IDE can effectively degrade insulin, amylin, and glucagon, pancreatic hormones that control blood glucose levels, as well as amyloid β (Aβ), a peptide implicated in Alzheimer’s disease. IDE is a 110 kDa zinc metalloprotease that readily dimerizes in solution (Kd =~ 10 nM). IDE has at least two major conformational states in its catalytic cycle; open-state IDE captures substrates and releases products while closed-state IDE performs catalysis. Within the IDE dimer, each IDE subunit consists of ~55 kDa N- and C-terminal domains, IDE-N and IDE-C.

Further 3D classification revealed three major conformations and structural models were built. We again applied IDE dimer-focused classification with signal subtraction of the IDE-FabH11-E dimer to refine each conformation separately, which improved the resolution significantly. The three apo-IDE structures derive from combinations of the IDE partial open (pO) and open (O) states. The three conformers have resolution limits which correlated well with their relative populations: O/pO (4.2 Å, 73%), O/O (6.5 Å, 16%), and pO/pO (6.9 Å, 11%). Furthermore, two subunits within O/O or pO/pO states have noticeable differences in the distance and buried surface between IDE-N and IDE-C and the dihedral angle. The IDE pO and O states differs from the pC and C states by 5 Å to 24 Å increases in the distance between D1 and D4 and 7° to 17° increases in the dihedral angle, respectively. These changes result in decreased buried surface between IDE-N and IDE-C in pO and O states. Open-state IDE has an opening just wide enough to capture its substrates, for example, insulin, TGF-α, and MIP-1α/β, allowing the IDE catalytic chamber to attract these substrates with high dipole moment via charge complementarity. Our cryoEM structures reveal that only open-state IDE can capture its prototypical substrate, insulin, and release cleaved products.

>AIKRIGNHITKSPEDKREYRGLELANGIKVLLISDPTTDKSSAALDVHIGSLSDPPNIAGLSHFLEHMLFLGTKKYPKENEYSQFLSEHAGSSNAFTSGEHTNYYFDVSHEHLEGALDRFAQFFLSPLFDESAKDREVNAVDSEHEKNVMNDAWRLFQLEKATGNPKHPFSKFGTGNKYTLETRPNQEGIDVRQELLKFHSAYYSSNLMAVVVLGRESLDDLTNLVVKLFSEVENKNVPLPEFPEHPFQEEHLKQLYKIVPIKDIRNLYVTFPIPDLQKYYKSNPGHYLGHLIGHEGPGSLLSELKSKGWVNTLVGGQKEGARGFMFFIINVDLTEEGLLHVEDIILHMFQYIQKLRAEGPQEWVFQELKDLNAVAFRFKDKERPRGYTSKIAGILHYYPLEEVLTAEYLLEEFRPDLIEMVLDKLRPENVRVAIVSKSFEGKTDRTEEWYGTQYKQEAIPDEVIKKWQNADLNGKFKLPTKNEFIPTNFEILPLEKEATPYPALIKDTAMSKLWFKQDDKFFLPKANLNFEFFSPFAYVDPLHSNMAYLYLELLKDSLNEYAYAAELAGLSYDLQNTIYGMYLSVKGYNDKQPILLKKIIEKMATFEIDEKRFEIIKEAYMRSLNNFRAEQPHQHAMYYLRLLMTEVAWTKDELKEALDDVTLPRLKAFIPQLLSRLHIEALLHGNITKQAALGIMQMVEDTLIEHAHTKPLLPSQLVRYREVQLPDRGWFVYQQRNEVHNNSGIEIYYQTDMQSTSENMFLELFAQIISEPAFNTLRTKEQLGYIVFSGPRRANGIQGLRFIIQSEKPPHYLESRVEAFLITMEKSIEDMTEEAFQKHIQALAIRRLDKPKKLSAESAKYWGEIISQQYNFDRDNTEVAYLKTLTKEDIIKFYKEMLAVDAPRRHKVSVHVLAREMDSCPVVGEFPCQNDINLSQAPALPQPEVIQNMTEFKRGLPLFPLVKPH[2x]> LAAVSVDCSEYPKPACTLEYRPLCGSDNKTYGNKCNFCNAVVESNGTLTLSHFGK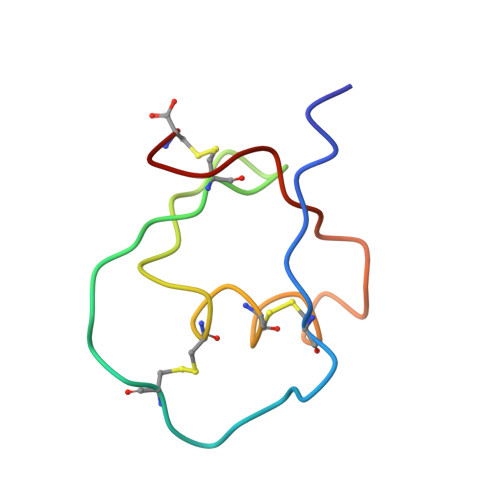C> MADTRIGVTIYKYDDNFMSVVRKAIEQDAKAAPDVQLLMNDSQNDQSKQNDQIDVLLAKGVKALAINLVDCAAAGTVIEKARGQNVPVVFFNKEPSRKALDSYDKAYYV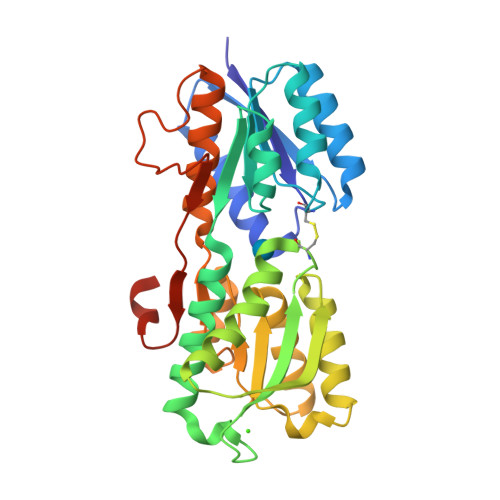GTDSKESGIIQGDLIAKHWAANQGWDLNKDGQIQFVLLKGEPCHPDAEARTTYVIKELNDKGIKTEQLQLDTAMWDTAQAKDKMDAWLSGPNANKIEVVIANNDAMAMGAVEALKAHNKSSIPVFGVDALPEALALVKSGALAGTVLNDANNQAKATFDLAKNLADGKGAADGTNWKIDNKVVRVPYVGVDKDNLAEFSKKGSHHHHHH>MRGSHHHHHHGLVPRGSMIRTMLQGKLHRVKVTHADLHYEGSCAIDQDFLDAAGILENEAIDIWNVTNGKRFSVYAIAAERGSRIISVNGAAAHCASVGDIVIIASFVTMPDEEAR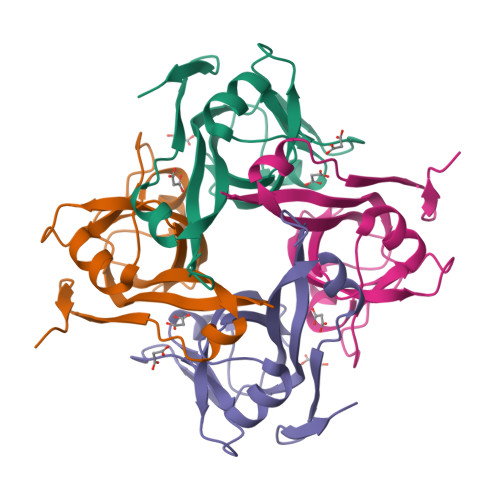TWRPNVAYFEGDNEMKRTAKAIPVQVA[2x]> TSTNATSSSC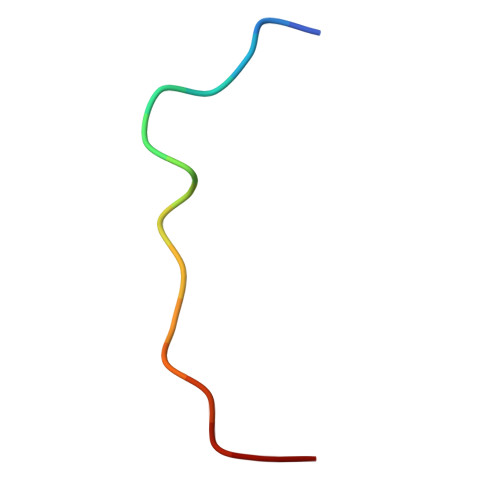ATPSLK>[2x]MEIPVIEPLFTKVTEDIPGAAGPVFDKNGDFYIVAPYVEVNGKPAGEILRIDLKTGKKTVICKPEVNGYGGIPAGCQCDRDANQLFVADMRLGLLVVQTDGTFEEIAKKDSEGRRMQGCAYCAFDYEGNLWITAPAGEVAPADFTISLQEKFGSIYCFTTDGQMIQVDTAFQXPAGIAVRHMNDGRPYQLIVAEQPTKKLWSYDIKGPAKIENKKVWGHIPGTHKGGAAGMDFDEDNNLLVANWGSSHIEVFGPDGGQPKMRIRCPFEKPSALHFKPQTKTIFVTEHENNAVWKFEWQRNGKKQYCETLKFGIFGSLEWSHPQFEK

Recently our laboratory has introduced a powerful mode of photochemistry into proteins, namely triplet energy transfer (EnT) photocatalysis, by developing an enantioselective [2 + 2] cyclase that relies on a genetically programmed benzophenone as a triplet sensitizer. Compared with benzophenones, thioxanthones have strong absorbance features that extend into the visible spectrum and are less susceptible to off-pathway processes that compromise EnT efficiency. Here, we develop engineered translation components to embed thioxanthone triplet sensitizers into proteins. This system enables the development of highly efficient and oxygen-tolerant photoenzymes that are powered by visible light and can achieve selective conversions that are beyond the reach of existing photocatalysts.

The resulting variant, VEnT1.0, shows appreciable levels of stereocontrol (85% e.e. for (+)-1a) and substantially improved activity compared with small-molecule thioxanthone as a sensitizer. To further improve enzyme performance, VEnT1.0 was subjected to three rounds of directed evolution. To gain further insights into the catalytic mechanism of VEnT1.3, crystal structures of apo-VEnT1.0 and apo-VEnT1.3 were solved at 1.5-Å and 1.8-Å resolution, respectively. The structures show that the mutations installed during evolution have resulted in a repositioning of the mTX sensitizer. The protein pocket extends the triplet lifetime in VEnT1.0 (τ2 = 6.9 µs) compared with free mTX (τ2 = 5.0 µs) under anaerobic conditions. Interestingly, the large fluorescence emission signal observed with free thioxanothone in aqueous buffer is substantially reduced in VEnT1.0 and VEnT1.3, suggesting that sensitizer confinement in a hydrophobic active site pocket facilitates intersystem crossing to the triplet state.>MGCGIMKYGITEMVKTIDTKTRVVDVTNEIAKKKYQAIRDFLEGEEFKEVVIFGVYLWGNYTAQMLSKYADKVYLVDIHEFMKGFVPNNNSIKFLNLNEFKLKFIRGEVNPDLIVDLTGLGGIEPEFLAKFNPKVFIVEDPKGVFDVDIYEADNTYKRTAPFIEKAKVGVLKT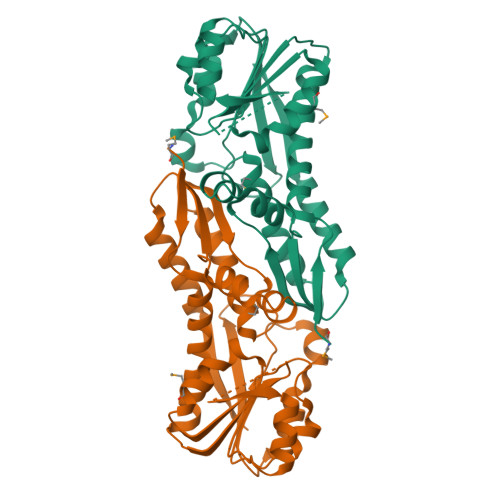YRKARVSKTSGTMTLTIDTIVDASREITSLDGVLYAIPNLRYYEGILFHENDIHKFLSEISQPAITISTLNDVLDEAEEILSNNINLIYSFVEEL[4x]RNA thermometers are non-coding RNAs found in the 5′ untranslated regions (5′-UTRs) of genes, where they regulate gene expression in response to changes in temperature. ROSE-like thermometers contain a conserved U(U/C)GCU motif that imperfectly base pairs with the Shine-Dalgarno (SD) sequence in a stem with a predicted bulged G nucleotide. Increases in temperature promote destabilization of the motif followed by exposure of the SD for ribosomal binding, resulting in increased gene expression. The oppF gene encodes an ATP-binding protein, which is one of the ABC domain components of the oligopeptide ABC transporter and is part of the opp operon.

Next, we investigated if the P2 stem of the P. stuartii oppF RNA thermometer can achieve thermoregulation by itself (Experimental procedures). Surprisingly, P2 alone exhibited an increased heat induction at 42 °C of ∼8.4-fold, showing that it is sufficient for complete thermoregulation. To further investigate the stereochemical consequences of the conserved ROSE-like motif, we determined the 2.7 Å-resolution X-ray crystal structure of the P2 stem using crystals grown at 21 °C. The elucidated structure is that of a dimer of P. stuartii oppF P2 RNA molecules, in which the two stems are distal from the fortuitous dimer interface. As predicted, G44 is bulged from the stem formed by the ROSE-like motif and the SD. At the crystallization temperature, a wobble (U43·G61) and a canonical (C45–G60) base pair adjacent to the bulged G44 maintains the two RNA strands together. The bulged G44 enhances the inability of U43 to stack with the succeeding nucleotide of the helix, C45, likely decreasing the stability of the stem and reducing its melting temperature. This is even more noticeable when considering the distance of the glycosyl carbon atoms C1′ of U43 and C45, measured at 7.6 Å, considerably higher than the average 5.5 Å of the rest of the C1′ atoms of the RNA molecule. In addition, the bulged G44 seems to exacerbate the helical twist angles between the two flanking base pairs, with the preceding U43·G61 being overwound at 40.7° and the succeeding C45–G60 being underwound at 26.7°. Combined, these structural features may play an important role in the destabilization of the stem at higher temperatures.

>AGCUUGCUUUAAGCCGCUGGAGGAGCU[2x]>MHRTSNGSHATGGNLPDVASHYPVAYEQTLDGTVGFVIDEMTPERATASVEVTDTLRARWGLVHGGAYCALAEMLATEATVAVVHEKGMMAVGQSNHTSFFRPVKEGHVRAEAVRIHAGSTTWFWDVSLRDDAGRL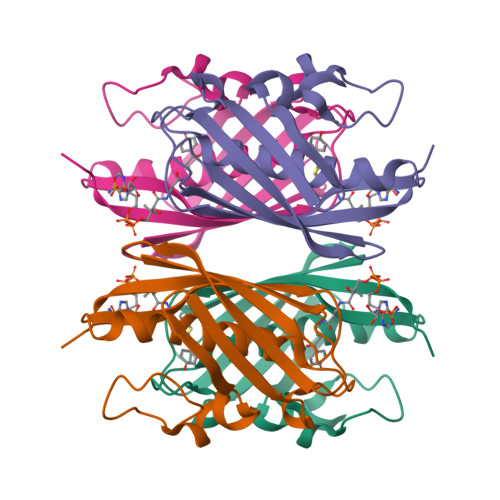CAVSSMSIAVRPRRD[2x]> MESKRNKPGKATGKGKPVGDKWLDDAGKDSGAPIPDRIADKLRDKEF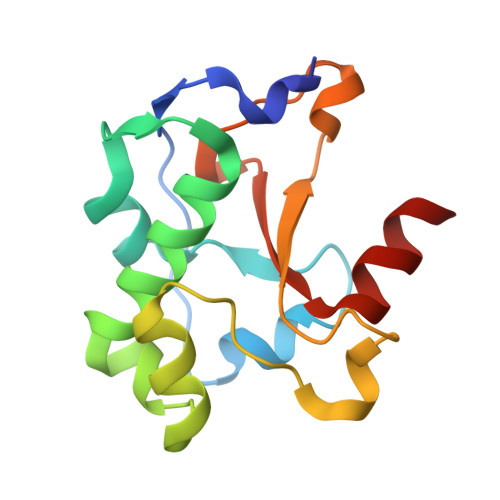KSFDDFRKAVWEEVSKDPELSKNLNPSNKSSVSKGYSPFTPKNQQVGGRKVYELHHDKPISQGGEVYDMDNIRVTTPKRHIDIHRGK>[6x]SMIEDIKGYKPHTEEKIGKVNAIKDAEVRLGLIFDALYDEF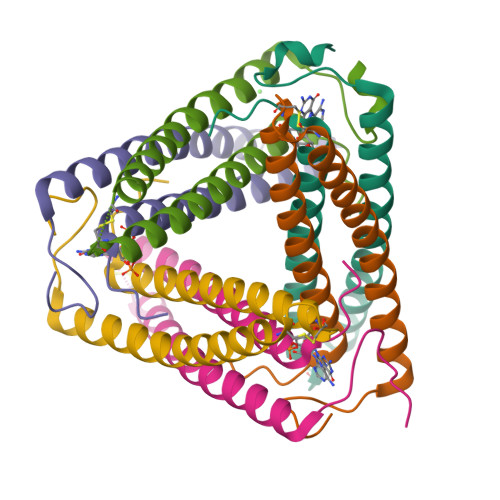WEALDNCEDCEFAKNYAESLDQLTIAKTKLKEASMWACRAVFQPEEKY>PIKVIEQQQREMKNAEDNEKKDIQNIVKLKVFDQSIKTEDFYVIDVNSYCKANGDYLIGEFTVTQFSLQDGVKNSYHETIIPSCVPVGYMFDVKLGAEEFGLEMPGTDDAGPNYIQILANIIDYLKQKDRTVQVLPPMFTLPEKVDAVQNFISQMCNCATEDDSLFRIYKLDTFFFTLINAISSHHDEGFPKESLALTQLTKDLFDYTPGIACERHESLDKSNVCTTSRVKRWVFTILDRCCPLLGIPLQPGKHLPFDYDI[4x]

Piwi-interacting RNAs (piRNAs) guide Piwi argonautes to their transposon targets for silencing. The highly conserved protein Maelstrom is linked to both piRNA biogenesis and effector roles in this pathway. Maelstrom is composed of an amino-terminal High Mobility Group (HMG) box and a predicted carboxy-terminal MAEL domain that is a signature feature of the protein across the animal kingdom (Zhang et al. 2008). Our studies suggest that the ancient MAEL nuclease domain evolved to function as an RNA-binding module in metazoan Maelstrom.

To explore this, we crystallized a fragment of Bombyx Maelstrom (BmMael) containing the MAEL domain. This reveals an α/β structure composed of an amino-terminal linker helix followed by the MAEL domain. The MAEL domain is composed of a central β-sheet composed of five strands (β1–β5), where β2 is antiparallel to the others. The β-sheet is flanked on one face by three helices (α8–α10) and on the other by two helices (α6 and α7). Despite this overall resemblance between MAEL and DEDD nuclease domains, one striking difference is the presence of a Zn2+ ion in the MAEL structure that bridges the bottom of the β-sheet and the loop connecting α9 and α10, which encompasses η2. The Zn2+ ion is tetrahedrally coordinated by E137 from β2, H293 from η2, and residues C290 and C302 from loops. The fact that the Zn2+ ion was captured from the bacterial culture media, and not added during initial crystallization trials, points to its paramount importance for the structural integrity of the MAEL domain. A closer comparison of the Bombyx MAEL domain with the DEDD nuclease domain in E. coli Pol III reveals that the catalytic residues (D12, E14, D103, and D167) essential for coordinating two Mn2+ ions in the bacterial enzyme are not conserved in the MAEL domain. Intriguingly, an extensive hydrogen bonding network links these inactive residues in the catalytic pocket: N124 from β1 forms hydrogen bonds (dotted black line in figure) with both E137 of the ECHC motif and R306 from α9, while R306 has an additional interaction with D122 from β1. Interestingly, the construct lacking the HMG box (containing only the linker helix plus the MAEL domain) also showed robust affinity for RNA (129.9 ± 18.86 nM).> GRLWLPNTPDASDPQRGRLAPPGELNLTTASVPMLRWYAERFCFVLVTTAEFPRDPGQLLYIPKTYLLGRPRNASLPELPEAGPTSRPPAEVTQLKG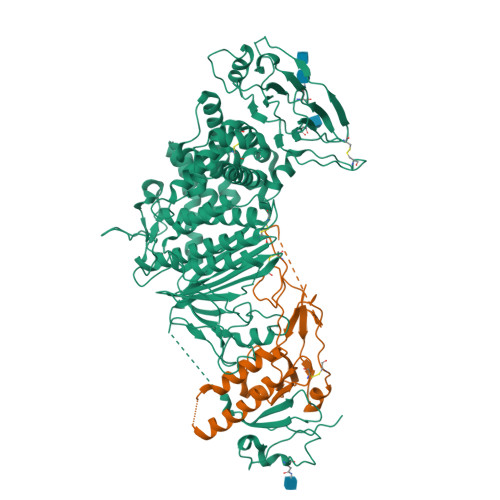LSHNPGASALLRSRAWVTFAAAPDREGLTFPRGDDGATERHPDGRRNAPPPGPPAGTPRHPTTNLSIAHLHNASVTWLAARGLLRTPGRYVYLSPSASTWPVGVWTTGGLAFGCDAALVRARYGKGFMGLVISMRDSPPAEIIVVPADKTLARVGNPTDENAPAVLPGPPAGPRYRVFVLGAPTPADNGSALDALRRVAGYPEESTNYAQYMSRAYAEFLGEDPGSGTDARPSLFWRLAGLLASSGFAFVNAAHAHDAIRLSDLLGFLAHSRVLAGLAARGAAGCAADSVFLNVSVLDPAARLRLEARLGHLVAAILEREQSLVAHALGYQLAFVLDSPAAYGAVAPSAARLIDALYAEFLGGRALTAPMVRRALFYATAVLRAPFLAGAPSAEQRERARRGLLITTALCTSDVAAATHADLRAALARTDHQKNLFWLPDHFSPCAASLRFDLAEGGFILDALAMATRSDIPADVMAQQTRGVASVLTRWAHYNALIRAFVPEATHQCSGPSHNAEPRILVPITHNASYVVTHTPLPRGIGYKLTGVDVRRPLFITYLTATCEGHAREIEPKRLVRTENRRDLGLVGAVFLRYTPAGEVMSVLLVDTDATQQQLAQGPVAGTPNVFSSDVPSVALLLFPNGTVIHLLAFDTLPIATIAPHHHHHH;> SQATEYVLRSVIAKEVGDILRVPCMRTPADDVSWRYEAPSVIDYARIDGIFLRYHCPGLDTFLWDRHAQRAYLVNPFLFAAGFLEDLSHSVFPADTQETTTRRALYKEIRDALGSRKQAVSHAPVRAGCVNFDYSRTRRCVGRRDLRPANTTSTWEPPVSSDDEASSQSKPLATQPPVLALSNAPPRRVSPTRGRRRHTRLRRN>GSHMASMKKKGSVVIVGRINLSGDTAYAQQTRGEEGCQETSQTGRDKNQVEGEVQIVSTATQTFLATSINGVLWTVYHGAGTRTIASPKGPVTQMYTNVDKDLVGWQAPQGSRSLTPCTCGSSDLYLVTRHADVIPVRRRGDSRGSLLSPRPISYLKGSAGGPLLCPAGHAVGIFRAAVSTRGVAKAVDFIPVESLETTMRS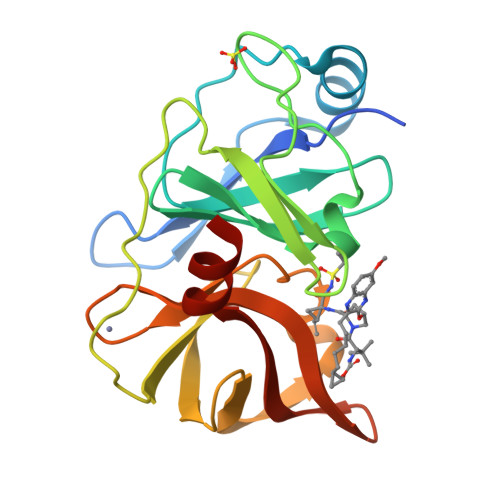P[4x]>[9x]MQLFDLS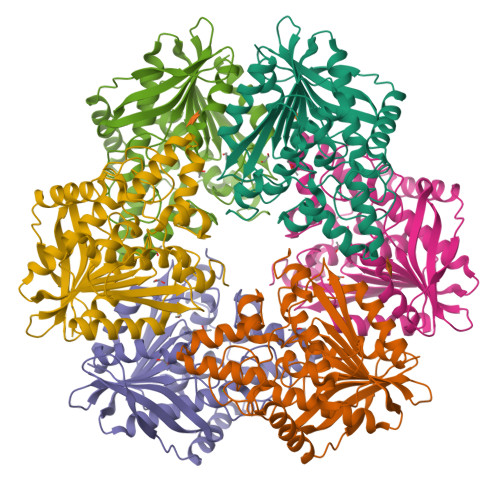LEELKKYKPKKTARPDFSDFWKKSLEELRQVEAEPTLESYDYPVKGVKVYRLTYQSFGHSKIEGFYAVPDQTGPHPALVRFHGYNASYDGGIHDIVNWALHGYATFGMLVRGQGGSEDTSVTPGGHALGWMTKGILSKDTYYYRGVYLDAVRALEVIQSFPEVDEHRIGVIGGSQGGALAIAAAALSDIPKVVVADYPYLSNFERAVDVALEQPYLEINSYFRRNSDPKVEEKAFETLSYFDLINLAGWVKQPTLMAIGLIDKITPPSTVFAAYNHLETDKDLKVYRYFGHEFIPAFQTEKLSFLQKHLLLST;>[3x]MQLFDLSLEELKKYKPKKTARPDFSDFWKKSLEELRQVEAEPTLESYDYPVKGVKVYRLTYQSFGHSKIEGFYAVPDQTGPHPALVRFHGYNASYDGGIHDIVNWALHGYATFGMLVRGQGGSEDTSVTPGGHALGWMTKGILSKDTYYYRGVYLDAVRALEVIQSFPEVDEHRIGVIGGXQGGALAIAAAALSDIPKVVVADYPYLSNFERAVDVALEQPYLEINSYFRRNSDPKVEEKAFETLSYFDLINLAGWVKQPTLMAIGLIDKITPPSTVFAAYNHLETDKDLKVYRYFGHEFIPAFQTEKLSFLQKHLLLST> TNLVAEPFAKLEQDFGGSIGVYAMDTGSGATVSYRAEERFP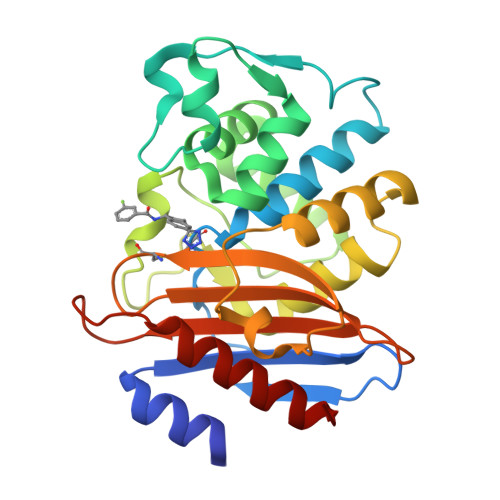LCSSFKGFLAAAVLARSQQQAGLLDTPIRYGKNALVPWSPISEKYLTTGMTVAELSAAAVQYSDNAAANLLLKELGGPAGLTAFMRSIGDTTFRLDRWELELNSAIPGDARDTSSPRAVTESLQKLTLGSALAAPQRQQFVDWLKGNTTGNHRIRAAVPADWAVGDKTGTCGVYGTANDYAVVWPTGRAPIVLAVYTRAPNKDDKHSEAVIAAAARLALEGLGV> ADANFRVLSQQLSRLNKTLAAGRPTINHPTFVGSERCRPGYTFTSITLKPPKIDRGSYYGKRLLLPDSVTEYDKKLVSRLQIRVNPLPKFDSTVWVTVRKVPASSDLSVAAISAMFADGASPVLVYQYAASGVQANNKLLYDLSAMRADIGDM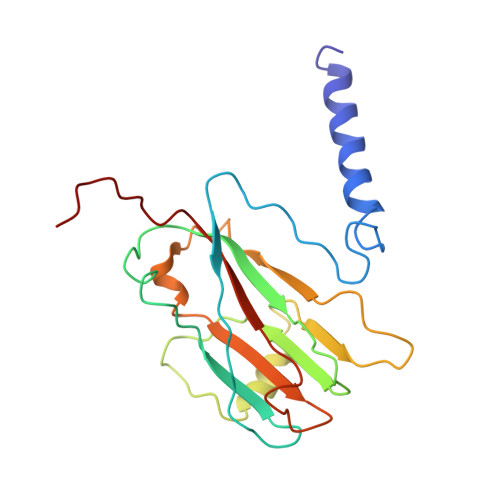RKYAVLVYSKDDALETDELVLHVDIEHQRIPTSGVLPV>MAVYHMTPPSGWLCNPQRPVTTHGAYQLYYLHSDQNNGPGGWDHASTTDGVAFTHHGTVMPLRPDFPVWSGSAVVDTANTAGFGAGAVVALATQPTDGVRKYQEQYLYWSTDGGFTFTALPDPVIVNTDGRAATTPAEIENAEWFRDPKIHWDTARGEWVCVIGRLRYAAFYTSPNLRDWTLRRNFDYPNHALGGIECPDLFEITADDGTRHWVLAASMDAYGIGLPMTYAYWTGTWDGEQFHADDLTPQWLDWGWDWYAAVTWPSIDAPE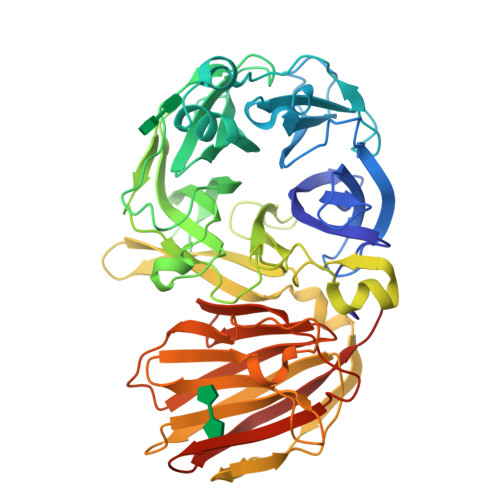TKRLAIAWMNNWKYAARDVPTDASDGYNGQNSIVRELRLARQPGGWYTLLSTPVAALTNYVTATTTLPDRTVDGSAVLPWNGRAYEIELDIAWDTATNVGISVGRSPDGTRHTNIGKYGADLYVDRGPSDLAGYSLAPYSRAAAPIDPGARSVHLRILVDTQSVEVFVNAGHTVLSQQVHFAEGDTGISLYTDGGPAHFTGIVVREIGQAILEHHHHHHHH[4x]>[2x]MHHHHHHMKEVVSSVYKEILVKLGLTEDRIETLEMKGGIIEDEFDGIRYVRFKDSAGKLRRGTVVIDEEYVIPGFPHIKRIINLRSGIRRIFKRGEFYVEE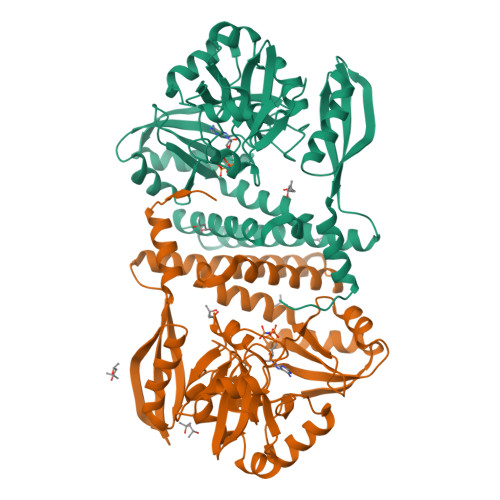KVDGYNVRVVMYKGKMLGITRGGFICPFTTERIPDFVPQEFFKDNPNLILVGEMAGPESPYLVEGPPYVKEDIQFFLFDVQEIKTGRSLPVEERLKIAEEYGINHVEVFGKYTKDDVDELYQLIERLSKEGREGIIMKSPDMKKIVKYVTPYANINDIKIGARVFYELPPGYFTSRISRLAFYLAEKRIKGEEFERVAKELGSALLQPFVESIFDVEQEEDIHELFKVRVKRIETAYKMVTHFEKLGLKIEIVDIEEIKDGWRITFKRLYPDATNEIRELIGGKAFVD> EDPEVLFKNKGCVACHAIDTKKVGPAYADVAKKYAGRKDAVDYLAGKIKKGGSGVWGSVPAPPQNVTDAEAKQLAQWILSIK;> NEQLAKQKGCMACHDLKAKMVGPAYKDVAAKFAGQAGAEAELAQRIKNGSQGV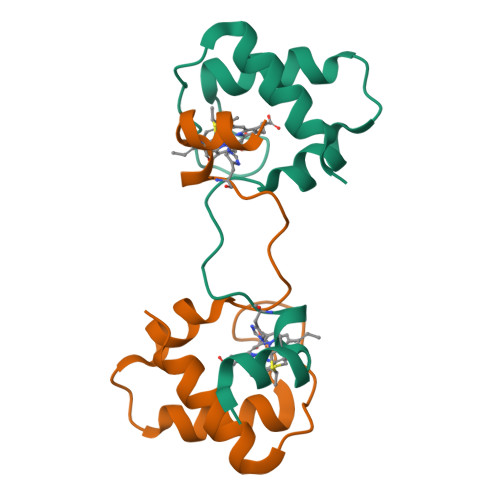WGPIPMPPNAVSDDEAQTLAKWVLSQK(3S)-6,8-dihydroxy-3-{[(2R,6S)-6-methyloxan-2-yl]methyl}-3,4-dihydro-1H-2-benzopyran-1-one 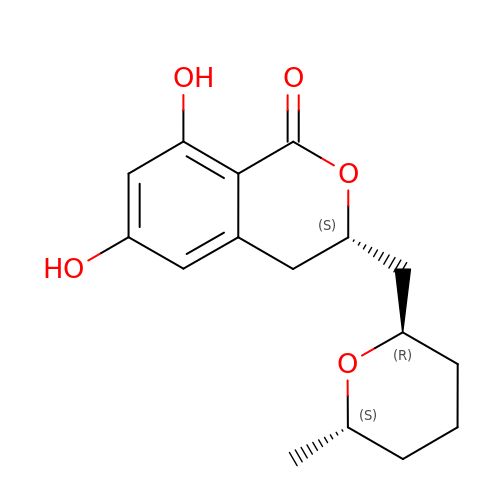| C16 H20 O5 | WOMKDMUZNBFXKG-BIMULSAOSA-N> MHHHHHHMKSIDEQSLHNARRLFESGDIDRIEVGTTAGLQQIHRYLFGGLYDFAGQIREDNISKGGFRFANAMYLKEALVKIEQMPERTFEEIIAKYVEMNIAHPFLEGNGRSTRIWLDLVLKKNLKKVVNWQNVSKTLYLQAMERSPVNDLELRFLLKDNLTDDVDNREIIFKGIEQSYYYGGYEKG

The ubiquitous FIC domain (pfam 02661) found in proteins of all domains of life and viruses has only recently been shown to confer ATase activity. The vast majority of Fic proteins are characterized by a conserved HxF[D/E]GNGRxxR active site motif and catalyses adenylylation, an enzymatic activity that involves nucleophilic attack of a target hydroxyl group onto the α-phosphate of ATP. Helices α4 and α5 are joined by a loop that together with the N-terminal cap of helix α5 forms the active center represented by a signature motif with the consensus sequence HxFx(D/E)GNGRxxR. For the comparative structure/function study on the inhibitory mechanism of Fic proteins from the various classes we chose as representatives the FIC domain of VbhT (residues 1 to 198) from Bartonella schoenbuchensis in complex with its cognate antitoxin VbhA (VbhA/VbhT(FIC); class I), Fic protein SO_4266 from Shewanella oneidensis (SoFic; class II) and Fic protein NMB0255 from Neisseria meningitidis (NmFic; class III).

In fact, a truncation mutant of the class III Fic protein from N. meningitidis (NmFic) lacking the entire C-terminal αinh helix showed strong ATase activity and allowed to study the catalytic and inhibitory mechanism in detail. To reveal the underlying inhibition relief mechanism, crystal structures of the three mutant proteins in complex with ATP or AMPPNP were determined to high resolution. For NmFicE186G this is not surprising, since the complex structure has been obtained by soaking and auto-adenylylation would require partial unfolding of αinh carrying the modifiable tyrosine (Y183). Since we do not see adenylylated residues, the extend of modifications may be either minor, locate to flexible loops or only the unmodified fraction may have crystallized. Figs. 3A–C show that in all three cases, the nucleotide is well resolved and, in contrast to the wild-type complexes, shows a unique conformation and relative position within the binding site. In all structures, the α- and β-phosphate moieties form four H-bonds with the four exposed backbone amide groups of the compound anion binding nest at the N-terminal end of helix α5. In all the structures, a magnesium ion is present albeit with high B-factor for NmFicE186G (63 Å2). Overall, the three structures display a unique mode of ATP binding that can be attained only in the mutants, since the γ-phosphate effectively adopts the position that is taken by the inhibitory glutamate in the wild-type proteins. Most relevantly, the reorganization of the triphosphate in the binding site results in a α-phosphate orientation that is now prone for in-line attack by an incoming target side-chain.>TDKRKDGSGKLLYCSFCGKSQHEVRKLIAGPSVYICDECV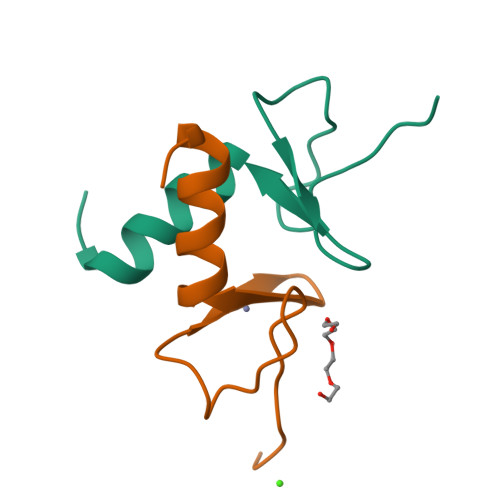DLCNDIIREEI[2x]> RAVPGGSSPAWTQCQQLSQKLCTLAWSAHPLVGHMDLREEGDEETTNDVPHIQCGDGCDPQGLRDNSQFCLQRIHQGLIFYEKLLGSDIFTGEPSLLPDSPV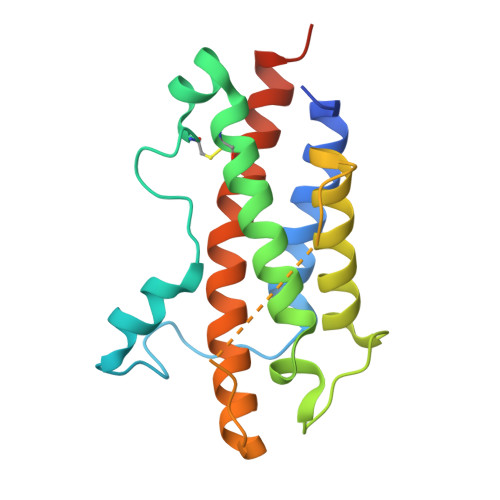GQLHASLLGLSQLLQPEGHHWETQQIPSLSPSQPWQRLLLRFKILRSLQAFVAVAARVFAHGAATLSPGTKHHHHHH> MAHHHHHHNPNYCFAGKTSSISDLKEVPRKNITLIRGLGHGAFGE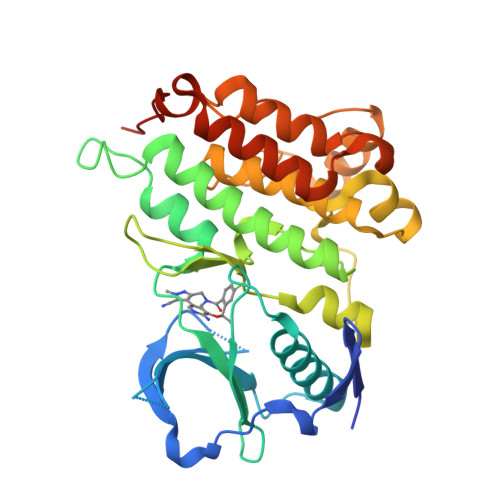VYEGQVSGMPNDPSPLQVAVKTLPEVYSEQDELDFLMEALIISKFNHQNIVRCIGVSLQSLPRFILLEFMAGGDLKSFLRETRPRPSQPSSLAMLDLLHVARDIACGCQYLEENHFIHRDIAARNCLLTCPGPGRVAKIGDFGMARDIYRASYYRKGGCAMLPVKWMPPEAFMEGIFTSKTDTWSFGVLLWEIFSLGYMPYPSKSNQEVLEFVTSGGRMDPPKNCPGPVYRIMTQCWQHQPEDRPNFAIILERIEYCTQDPDVINTALPIEYGPLVEEEEKV N-[1-(piperidin-4-yl)-1H-indol-5-yl]thiophene-2-carboximidamide 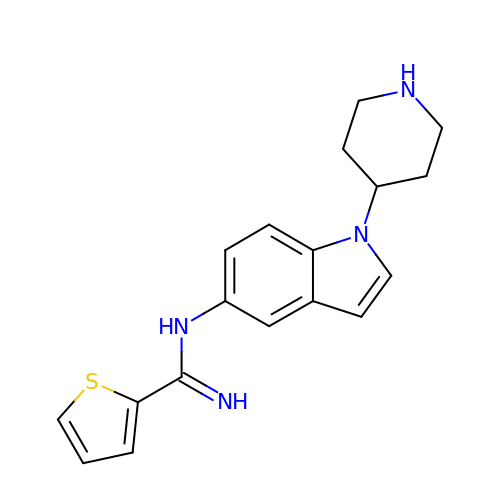| C18 H20 N4 S | XLCWIOAUURXLIX-UHFFFAOYSA-N> FACKTANGTAIPIGGGSANVYVNLAPVVNVGQNLVVNLSTQIFCHN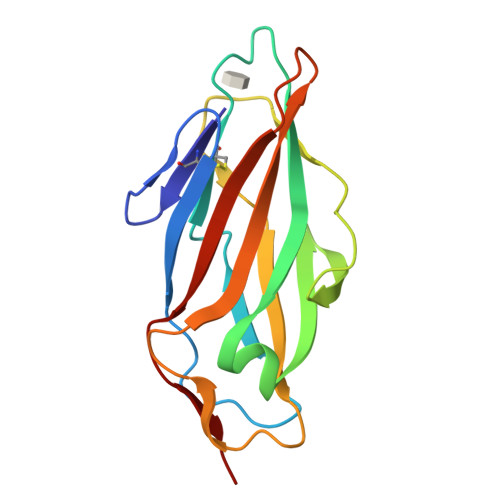DYPETITDYVTLQRGSAYGGVLSNFSGTVKYSGSSYPFPTTSETPRVVYNSRTDKPWPVALYLTPVSSAGGVAIKAGSLIAVLILRQTNNYNSDDFQFVWNIYANNDVVVPT>[8x]MIVSFMVAMDENRV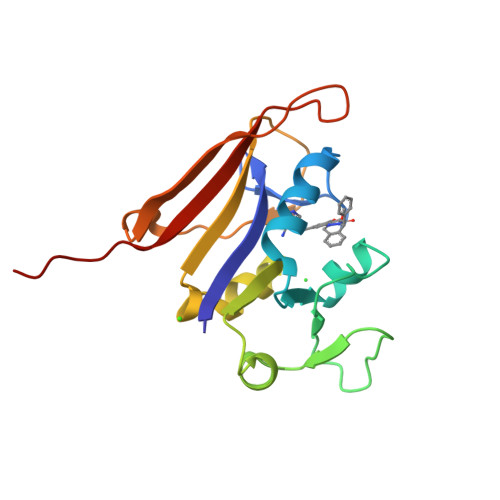IGKDNNLPWRLPSELQYVKKTTMGHPLIMGRKNYEAIGRPLPGRRNIIVTRNEGYHVEGCEVAHSVEEVFELCKNEEEIFIFGGAQIYDLFLPYVDKLYITKIHHAFEGDTFFPEMDMTNWKEVFVEKGLTDEKNPYTYYYHVYEKQQLVPR>HHHHHHMASSAQDGNNPLFSPYKMGKFNLSHRVVLAPMTRCRALNNIPQAALGEYYEQRATAGGFLITEGTMISPTSAGFPHVPGIFTKEQVREWKKIVDVVHAKGAVIFCQLWHVGRASHEVYQPAGAAPISSTEKPISNRWRILMPDGTHGIYPKPRAIGTYEISQVVEDYRRSALNAIEAGFDGIEIHGAHGYLIDQFLKDGINDRTDEYGGSLANRCKFITQVVQAVVSAIGADRVGVRVSPAIDHLDAMDSNPLSLGLAVVERLNKIQLHSGSKLAYLHVTQPRYVAYGQTEAGRLGSEEEEARLMRTLRNAYQGTFICSGGYTRELGIEAVAQGDADLVSYGRLFI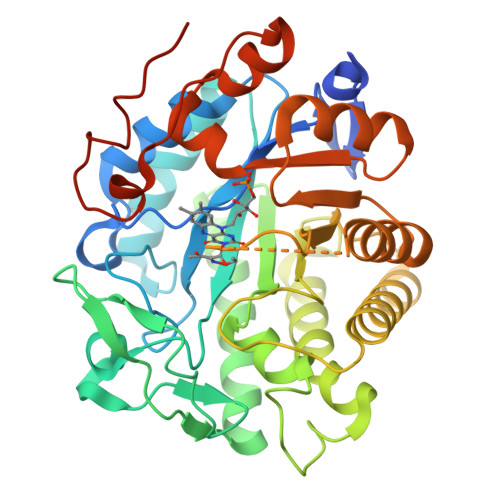SNPDLVMRIKLNAPLNKYNRKTFYTQDPVVGYTDYPFLQGNGSNGPLSRL[2x]>MKQYLELMQKVLDEGTQKNDRTGTGTLSIFGHQMRFNLQDGFPLVTTKRCHLRSIIHELLWFLQGDTNIAYLHENNVTIWDEWADENGDLGPVYGKQWRAWPTPDGRHIDQITTVLNQLKNDPDSERIIVSAWNVGELDKMALAPCHAFFQFYVADGKLSCQLYQRSCDVFLGLPFNIASYALLVHMMAQQCDLEVGDFVWTGGDTHLYSNHMDQTHLQLSREPRPLPKLIIKRKPESIFDYRFEDFEI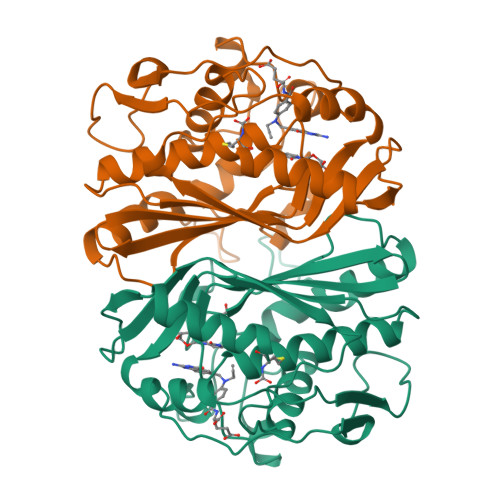EGYDPHPGIKAPVAI[2x]> MSSSVCPSDNTHATGAALQKILDYKKGDHQIMAGYFRSWRDTASGTGNKVSMLDLPDCLDIAFVFPEGDETASFWTTLKDTYVPALHGRGIKVVRSVGIAQLINTAWDNTPAGWQGLADALMKTVDDYGLDGLDIDVEQSLNANQLKQATGVFN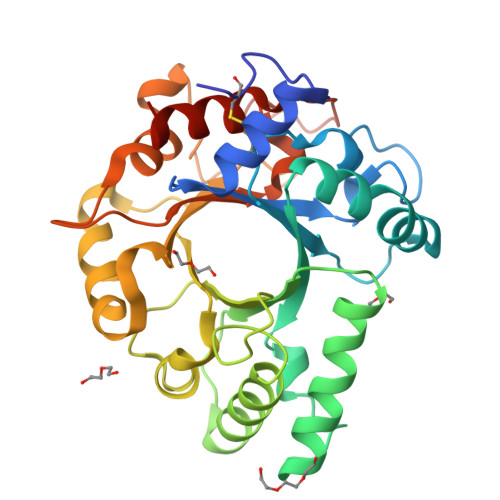ALAKKLGPKSGTGKLLIFDTNMDGTQPLWRNVYPTISYVLIQSYGRSISGLQTTYNSFKSYISSKQYLIGFSFYEENGTNWGDTTTPMTSSRAWQYAKWQPSGATKGGIFSYAIDRDGVAIGDNTLKTTDFTWTRQLIGAMNPHHHHHH>MKLDIKKTFSNRSDRVKGIDFHPTEPWVLTTLYSGRVEIWNYETQVEVRSIQVTETPVRAGKFIARKNWIIVGSDDFRIRVFNYNTGEKVVDFEAHPDYIRSIAVHPTKPYVLSGSDDLT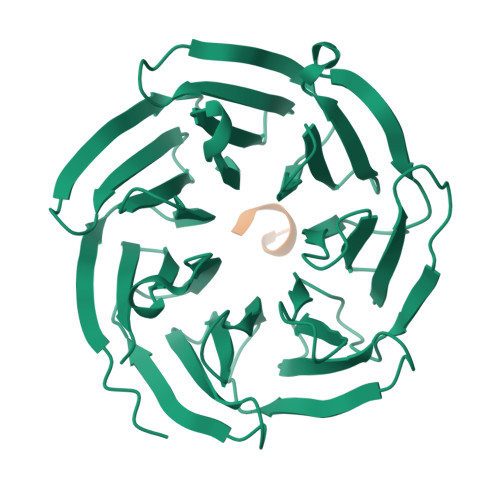VKLWNWENNWALEQTFEGHEHFVMCVAFNPKDPSTFASGCLDRTVKVWSLGQSTPNFTLTTGQERGVNYVDYYPLPDKPYMITASDDLTIKIWDYQTKSCVATLEGHMSNVSFAVFHPTLPIIISGSEDGTLKIWNSSTYKVEKTLNVGLERSWCIATHPTGRKNYIASGFDNGFTVLSLG[2x];>[2x]TFKKTN> GSHMSNITYVKGNILKPKSYARILIHSCNCNGSWGGGIAYQLALRYPKAEKDYVEVCEKYGSNLLGKCILLPSYENSDLLICCLFTSSFGGSSHGEKQSILNYTKLALDKLKTFREAKDKTRTSEDSIGDYLNGHIKYPIGEYKLEMPQINSGIFGV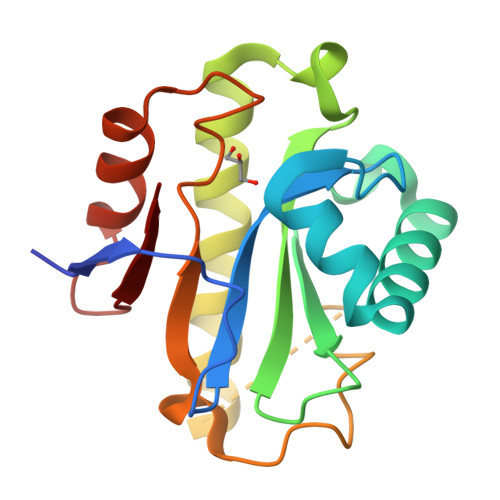PWKETERVLEEFSGDMSFTVYQL>MSDQSGKLLTSVRTYQGISPKLGERVFVDRSSVIIGDVELGDDCSVWPLAVIRGDMHHIRIGA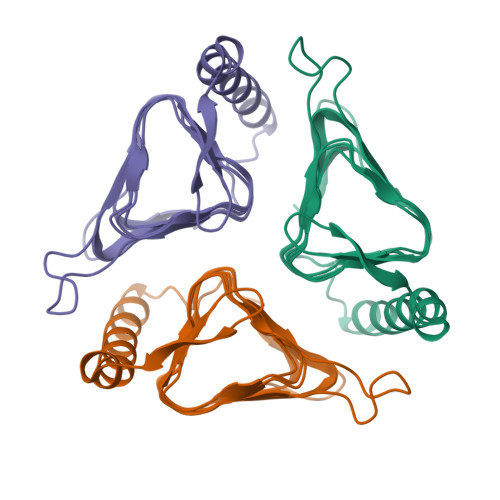RTSVQDGSVLHITHASDYNPGGYPLIIGDDVTIGHQAMLHGCTIGNRVLIGMKSMIMDGAIVEDEVIVAAGATVSPGKVLESGFVYMGTPAKKVRPITEKERSFFTYGAGNYVRLKDKHLAEGYDR[3x]> GPMTTTERPDLAWLDEVTMTQLERNPYEVYERLRAEAPLAFVPVLGSYVASTAEVCREVATSPDFEAVITPAGGRTFGHPAIIGVNG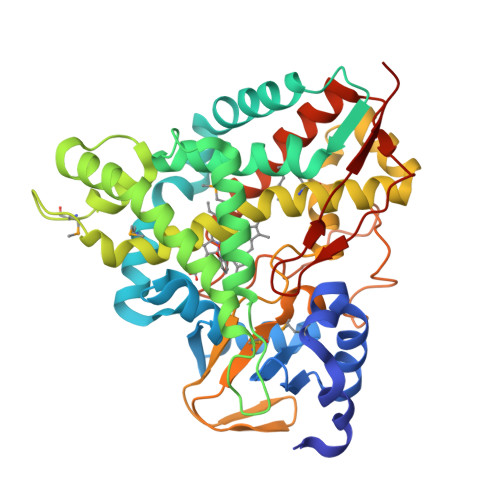DIHADLRSMVEPALQPAEVDRWIDDLVRPIARRYLERFENDGHAELVAQYCEPVSVRSLGDLLGLQEVDSDKLREWFAKLNRSFTNAAVDENGEFANPEGFAEGDQAKAEIRAVVDPLIDKWIEHPDDSAISHWLHDGMPPGQTRDREYIYPTIYVYLLGAMQEPGHGMASTLVGLFSRPEQLEEVVDDPTLIPRAIAEGLRWTSPIWSATARISTKPVTIAGVDLPAGTPVMLSYGSANHDTGKYEAPSQYDLHRPPLPHLAFGAGNHACAGIYFANHVMRIALEELFEAIPNLERDTREGVEFWGWGFRGPTSLHVTWEV> MNMISRRKNAKALSGAVTALILVIASVIIALVVVGFAFGLFGAFTGQGTVTQVGTATLSAGTGTLTVTLKNTGAATQVTGAIINGNAASVSGQVTISAGQNTYSISLGGISSSTLQNLVGSTISLTLQ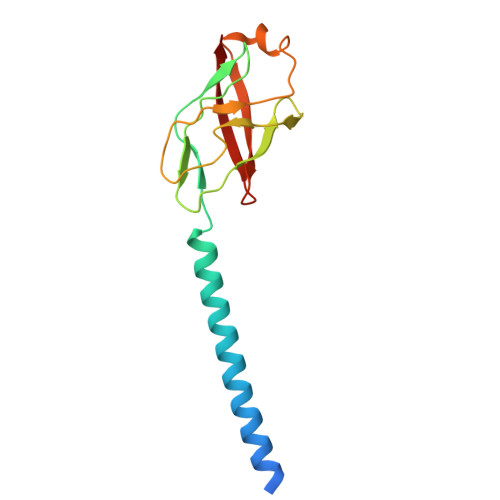LSNGQTVTVSAIITS>MNQYVNDPSNYQLLIKNLLFSPVAFNPEQEIVYANHRRHSYKTFHDRVRQFANALTKMGVKKGDTVAVMDYDSHRYLECYFAIPMIGAKLHMINVRLSPEQILYTIDHAEDDIILIHEEFLPILDQIKGRIDTVTRYVVLRDDEECEYERLLEQESTEYNFPDFDENTVATTFYTTGTTGFPKGVFFTHRQLVLHTMGILSTIGTNASQGRLHQGDIYMPITPMFHVHAWGLPYMATMLGVKQVYPGKYVPDVLLNLIEQEKVTFSHCVPTILHLLLSSPKSKAMDFSGWKVVIGGAALPKALCKSALERDIDVFAGYGMSETGPILSIVQLTPEQLELDVDQQAEYRSKTGKKVALVEAYIVDEDMNKLPHDGETAGEIVVRAPWLTPNYYKDNKNSKALWRGGYLHTGDVAHIDDEGFIKITDRVKDMIKISGEWVSSLELEDILHQHQSVSEVAVIGMPHNKWGEVPLALVTLKEDAQVTEKELLGFAKDFINKGILAREALLLKVKIVDEIA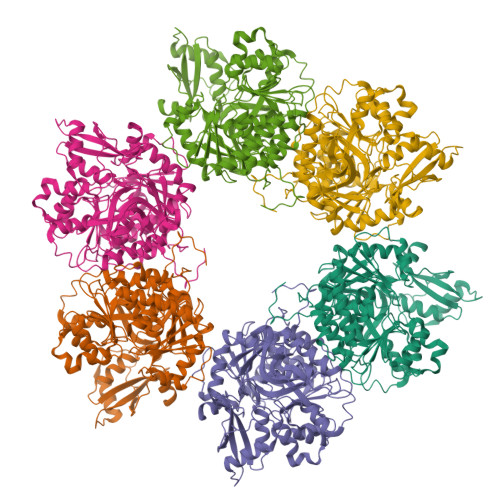KTSVGKVDKKELRKLHL[6x]> LAAMKNFAEQYAKRTDTYFCSDLSVTAVVIEGLARHKEELGSPLCPCRHYADKEAEVKNTFWNCPCVPMRERKECHCMLFLTPDNDFAGDAQGIPMETLEEKKA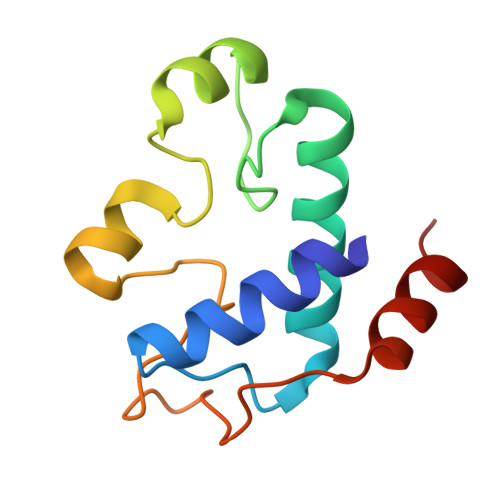SMA N~2~-{[2-chloro-3-(2-methylpyridin-3-yl)-1-benzothiophen-5-yl]carbamoyl}-N-(3-{methyl[(3R)-1-(5H-pyrrolo[2,3-d]pyrimidin-4-yl)piperidin-3-yl]amino}propyl)glycinamide 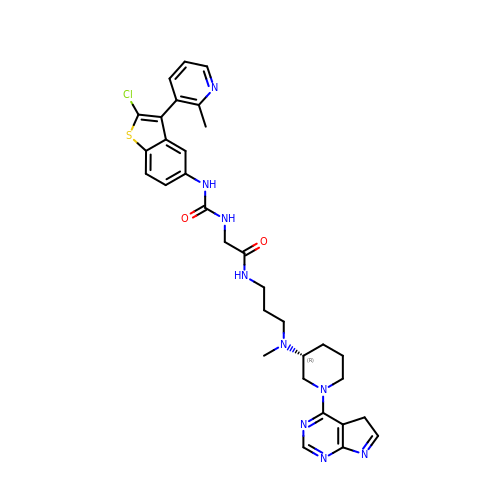| C32 H36 Cl N9 O2 S | BUHUWDQAOUQQHQ-JOCHJYFZSA-N>[22x]MCPTLNNIVSSLQR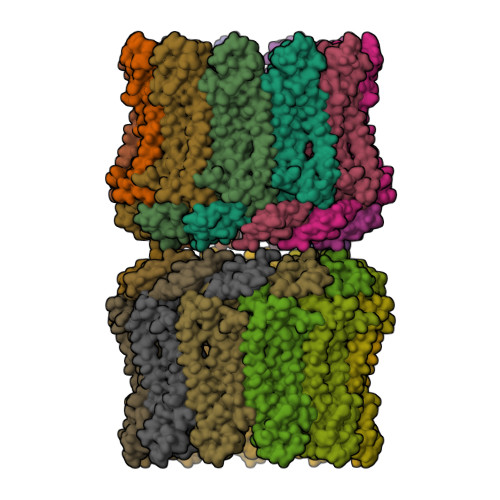NGIFINSLIAALTIGGQQLFSSSTFSCPCQVGKNFYYGSAFLVIPALILLVAGFALRSQMWTITGEYCCSCAPPYRRISPLECKLACLRFFSITGRAVIAPLTWLAVTLLTGTYYECAASEFASVDHYPMFDNVSASKREEILAGFPCCRSAPSDVILVRDEIALLHRYQSQMLGWILITLATIAALVSCCVAKCCSPLTSLQHCYWTSHLQNERELFEQAAEQHSRLLMMHRIKKLFGFIPGSEDVKHIRIPSCQDWKDISVPTLLCMGDDLQGHYSFLGNRVDEDNEEDRSRGIELKP>MGVKTFQFPFAEQLEKVAEQFPTFQILNEEGEVVNEEAMPELSDEQLKELMRRMVYTRILDQRSISLNRQGRLGFYAPTAGQEASQIASHFALEKEDFILPGYRDVPQIIWHGLPLYQAFLFSRGHFHGNQIPEGVNVLPPQIIIGAQYIQAAGVALGLKMRGKKAVAITYTGDGGTSQGDFYEGINFAGAFKAPAIFVVQNNRFAISTPVEKQTVAKTLAQKAVAAGIPGIQVDGMDPLAVYAAVKAARERAINGEGPTLIETLCFRYGPHTMSGDDPTRYRSKELENEWAKKDPLVRFRKFLEAKGLWSEEEENNVIEQAKEEIKEAIKKADETPKQKVTDLISIMFEELPFNLKEQYEIYKEKESK[4x];>MAQMTMVQAITDALRIELKNDPNVLIFGEDVGVNGGVFRATEGLQAEFGEDRVFDTPLAESGIGGLAIGLALQGFRPVPEIQFFGFVYEVMDSICGQMARIRYRTGGRYHMPITIRSPFGGGVHTPELHSDSLEGLVAQQPGLKVVIPSTPYDAKGLLISAIRDNDPVIFLEHLKLYRSFRQEVPEGEYTIPIGKADIKREGKDITIIAYGAMVHESLKAAAELEKEGISAEVVDLRTVQPLDIETIIGSVEKTGRAIVVQEAQRQAGIAANVVAEINERAILSLEAPVLRVAAPDTVYPFAQAESVWLPNFKDVIETAKKVMNF[4x];>MAFEFKLPDIGEGIHEGEIVKWFVKPGDEVNEDDVLCEVQNDKAVVEIPSPVKGKVLEILVPEGTVATVGQTLITLDAPGYENMTFKGQEQEEAKKEEKTETVSKEEKVDAVAPNAPAAEAEAGPNRRVIAMPSVRKYAREKGVDIRLVQGTGKNGRVLKEDIDAFLAGGAKPAPAAAEEKAAPAAAKPATTEGEFPETREKMSGIRRAIAKAMVHSKHTAPHVTLMDEADVTKLVAHRKKFKAIAAEKGIKLTFLPYVVKALVSALREYPVLNTSIDDETEEIIQKHYYNIGIAADTDRGLLVPVIKHADRKPIFALAQEINELAEKARDGKLTPGEMKGASCTITNIGSAGGQWFTPVINHPEVAILGIGRIAEKPIVRDGEIVAAPMLALSLSFDHRMIDGATAQKALNHIKRLLSDPELLLMEA[2x]

Pyruvate dehydrogenase (PDH) is a multienzyme complex that catalyzes the oxidative transformation of pyruvate to acetyl coenzyme A (CoA), CO2, and reducing equivalents in the form of NADH. The first step involves decarboxylation of pyruvate, which proceeds through formation of a covalent intermediate with the thiamine diphosphate cofactor (ThDP) in the active site of the pyruvate decarboxylase subunit (E1p; EC 1.2.4.2). E1p also catalyzes the second reaction step in which the acetyl group is transferred regiospecifically onto one of the sulfur atoms of a lipoyl moiety. The E1p enzyme from pyruvate dehydrogenase is a prototypical thiamine-dependent decarboxylase subunit from the extensive family of 2-oxo acid dehydrogenases.

The initial stage of catalysis is represented by the structure of E1p/E2p-PSBD with bound pyruvate. The reaction does not proceed because the cofactor has been replaced with the derivative 3-deazaThDP (thiamine diphosphate derivative where the N3 in the thiazolium ring is replaced with carbon) that mimics the ylide form but is unable to react with substrate. Pyruvate was soaked for several days into the cocrystals of E1p and 3-deazaThDP, and this resulted in density in the active-site pocket that is likely to be due to pyruvate binding (seeFigure 2 for location with respect to the whole structure). Although four copies of the active site occupy the crystal asymmetric unit, the density for the putative pyruvate is found in only two. In the remaining two sites, well-defined water molecules occupy the corresponding position. In one preferred orientation, the Cα carbon of the pyruvate is roughly 3.7 Å from C2 of 3-deazaThDP, its potential reaction partner, and is off the plane of the thiazole ring. The imidazole Nɛ of H128β contacts the pyruvate 2-oxo atom, one of the carboxylate oxygen atoms and the keto carbon of the pyruvate. The interaction with Nɛ of H128β might help to distinguish pyruvate from other carboxylic acids that lack the 2-oxo group. In the pyruvate-E1p cocrystals, the inner loops are ordered but the outer loops are not, again for all four subunits in the asymmetric unit. The pyruvate complex is not in an optimal geometry for the ThDP C2 to attack the pyruvate, and it is clear that either the substrate would have to be reorientated, or the thiazolium ring would have to tip substantially.>GAVELLVFNFLLILTILTIWLFKNHRFRFLHETGGAMVYGLIMGLILRYATAPTDIESGTVYDCGKLAFSPSTLLINITDQVYEYKYKREISQHNINPHLGNAILEKMTFDPEIFFNVLLPPIIFHAGYSLKKRHFFQNLGSILTYAFLGTAISCIVIGLIMYGFVKAMVYAGQLKNGDFHFTDCLFFGSLMSATDPVTVLAIFHELHVDPDLYTLLFGESVLNDAVAIVLTYSISIYSPKENPNAFDAAAFFQSVGNFLGIFAGSFAMGSAYAVVTALLTKFTKLCEF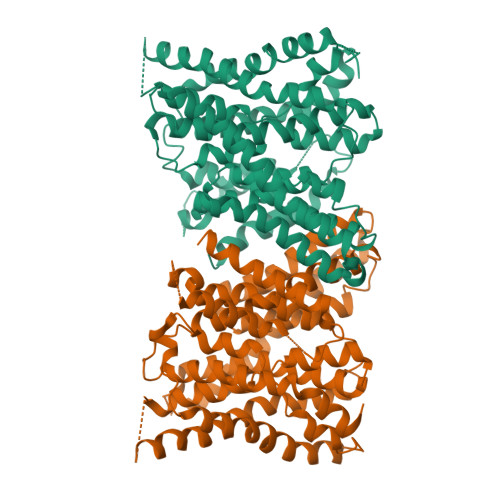PMLETGLFFLLSWSAFLSAEAAGLTGIVAVLFCGVTQAHYTYNNLSLDSKMRTKQLFEFMNFLAENVIFCYMGLALFTFQNHIFNALFILGAFLAIFVARACNIYPLSFLLNLGRKHKIPWNFQHMMMFSGLRGAIAFALAIRDTESQPKQMMFSTTLLLVFFTVWVFGGGTTPMLTWLQI[2x]> GQDVDKDPGRGLPVEEYHYGMQLDVKNVLHRTDNSTRTGVVP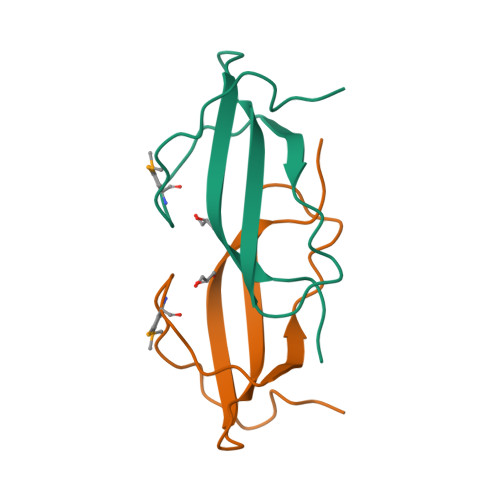VTVVYEDHSGELHKIRFLEWGGSTSNG> STQAAPLIS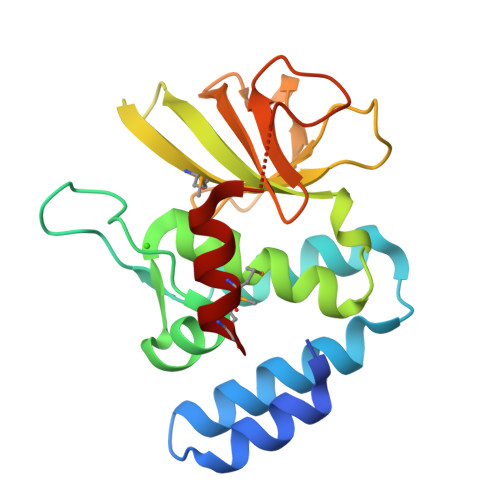VEKIQKLAQSYQGDTRKRFTAWGNLIDSLKKKPVKIQLEKVNSFFNQFNYETDPITGASDDYWKSPVEFIVDGGGDCEDFAIIKYFTLVAVGVPSDQLRITYAASLTLNQAHMVLSFYPTPESEPLILDSLESKILKASARPDLKPVYSFNAEGLWLAKTRGESSLMGDSKSLGKWDALMKRME> IIGGRESRPHSRPYMAYLQIQSPAGQSRCGGFLVREDFVLTAAHCWGSNINVTLGAHNIQRRENTQQHITARRAIRHPQYNQRTIQNDIMLLQLSRRVRRNRNVNPVALPRAQEGLRPGTLCTVAGWGRVSMRRGTDTLREVQLRVQRDRQCLRIFGSYDPRRQICVGDRRERKAAFKGDSGGPLLCNNVAHGIVSYGKSSG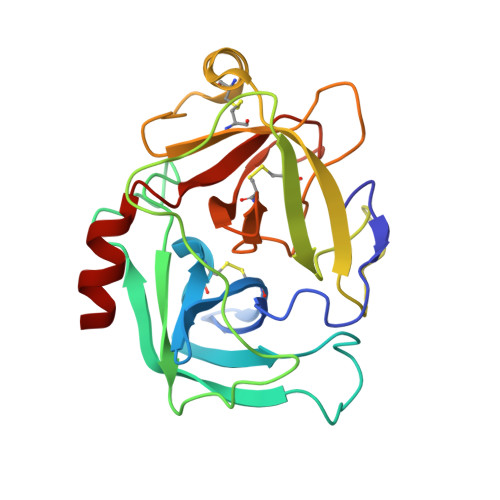VPPEVFTRVSSFLPWIRTTMR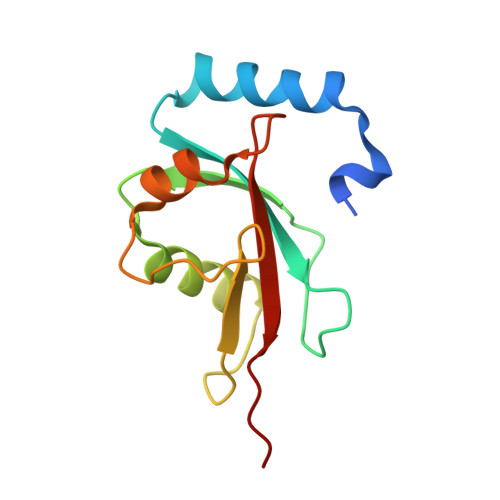> GPHMKSTFKSEYPFEKRKAESERIADRFPNRIPVICEKAEKSDIPEIDKRKYLVPADLTVGQFVYVIRKRIMLPPEKAIFIFVNDTLPPTAALMSAIYQEHKDKDGFLYVTYSGENTFG> MGSSHHHHHHSQDPMEIDELTALGGLLANIGKPVQRAGLYSGDHSTQGARFLRDLAENTGRAEYELLSLFSEFHHKGHMKNDELMIRRIKELSPERFGLTMEDVLNALWIVYEADNLASGEREEGQPQASRPLYSVFNPGKAYPWAELDFEKELPVPGDVFSIRSQDYRELVKRLWEELSKAKLRSDRLLPVLEKYLTFVSSVTSEGNIISLYDHMRMTSAIALAMLRAGCTAEDVRSGRCRKEKRFLLIEGDFSGIQDFIYRVSGKGTLKYLRARSAYLELIGWDVVLEILSRLGLTRANVVFNAGGHFMIIAQNTPDAVKELEEIRAKAVEWLYREFESDLYLAIEWEPVSGREFGREGGKNLFAEARKRLKHKLTVRKLKRFGEIKGLFEHGHTERLAECPVCGRELPEGKLEPSASDPETKVCPTCNRLVSLGGNLPKLLGFGRTAKNDAGVLVEGPFSGFVPYLQGGRPVGEQILVKNTLNPGEIPESAQFVPYFVADYFKKDPKGGVATFEELSMASTGTRRLGVMKGDVDRLGEFFSSMDSPSKLATASRFMDYFFKGYIGAIIEGKFGYIIGDVPSLRDWPEEPDIVVVYAGGDDFFIVGAWDQIFELAFRVRRAFNAYTGGKLTLSVGLGYFDERTPIYRMADVVSERLDTAKDEGRNRVFVVGRSRPLDGKHKLSYEWNHYEELWRTYAPRIYAGNGRLKGKLESKKGLLWKLLEIRELYVRDPNDVRWAYLTAYLLGRHGLSDLFPELVGIDTKAVERKEPQPVYWVDGVLKIVLMAVRR;>SMAYHQKHGGYGRGGYGRQDRPQVDASRLFGESPDVVGIKKMLEGKGKQWEAIQPYFDNVVREAKNFLEWSPNKRLANAVTVAAYLTSQGLKTNQVRKILDMARTTELKVKRGEGDIKDDLVKMRYLLAYTVGKATGQSKYSLDAFHRILDPMLEVLMGSPKKENFEKFYDFLQAVVAYHKFFGGGD[2x];>[3x]SMDRRFYGKIVIKGKIKAVTGLHIGSQRDISEIGGIANPVIKDPHTGLPYIPGSSLKGRLRSLFEILVNSRLGEWREKYPSLANYSPGSCRPDNQENCGKFFNRKINRGWIHVCPDYETALACPVCRLFGASGKESNFPSRIIVRDAFLTKEWEEKWRAGEAITEAKIEVGIDRVTSQANPRTNERVVAGAEFEFEIIYNVENTTHWRDDIKNLLTAMALLEDSYLGGSGSRGYGKVKFIFDSFEFRPLDYYRTGKDEDIVSIDAREKSVSDILSGFDSLFSEVEGKLEAG;> MPKFIAVKLIPKGPFRDIPRADTLFGAIGNAISAIHGQSAVEELVDAFVGGARISSAFPYSGDTYYLPKPLSVEPALEGILTGLDEEERYTTAKRLRKAKYLDLKNFELALRLRPFTIPEEIPYARVDVPRVVLDRVTQDSSIYFWEEIRFREKSGVYFLYSGPREVFDGYIAPAMRFLGDTGIGGKSTWGAGLFEVEFHEMKIDAPGSEYSVTLSNALPTKTPVLWRLLRKGGWS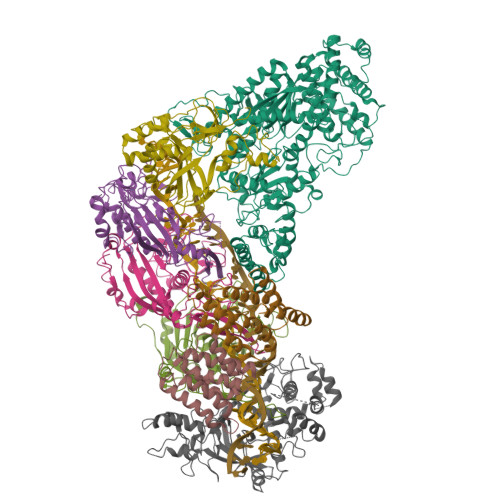FGRRKPRMTFIAEGSIVKNDPGGMERLELGLSHEVYVYGLTFPLGVELPEGLE;> MTERTLKVLSPLHIGTGNELTPVDIYPRENIIHVLDTERLVNDLMNLGVELNEILALLKNPPGDAYIWKGYIEEFHLDPSDYSIYTLKIHGKIGRKSMQIKEFIKLNGRPYIPGSSLKGAIRTAVLYKALKECGDARAVMRVVSKVNGDVARDIGRSEDVLDYYMSFLSRARIDRKRADDLLEAIVFGMEPDRRSKIRYEPKRDPMKALIVRDSKPVGRKHLAVYHVEVIGNPQPIPIWVEAIEPGAATDVEIHVDTEALRLNADYFNGLLWECLKERGEPGEVFEDFLWEAVDEFYTAVMKYETIEVQKFGRYTSQVRSFYASLEDHSGHVLRLGWGSGWLAMTIGLLLVEKGYKWENVRKKLGLGKKPGGSGFSREFPKTRRLADGMPMGWVVLEHHHHHH> MNNSGTIETSQSVDRVTHKILIDGSEIPGTYQVKSIQVTKEVNRIPTARLVILDGDAAERDFKVSNSDHFVPGKEIEITVGYHSDDETIFKGVVIRQNLKIRNNQSILIVESRDMAVKMTLRRKSKYFYELSDSDILEELISNHGLEADVASTENQHTELVQYDVTDWDFMMLRLQANGLLCLVDDGKVSIQKPDLSSEALETVTFGATILEFDAEMDARNQLPKVVSQAWNMSDQELLEKEGVDPSLETNGNISSSDLASLFDQEEEVLRHGGSKKDGSLQEWANAK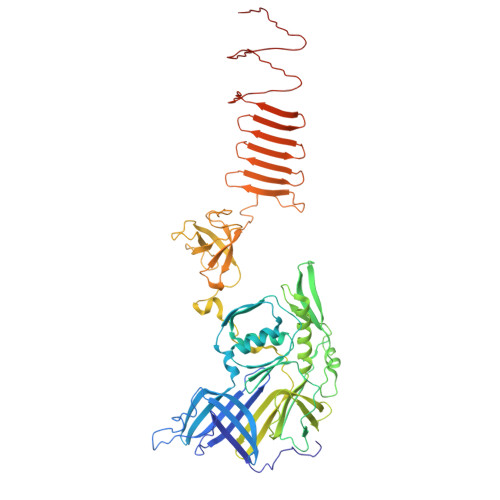WTFQQLAKTRGRIKFQGIPTVKPGVNLLLEGVGDRFNGKVFITGVNHQISEGNWTVDAQFGLNPEWFSESESNIHTPPAAGLTAAISGLHVGLVTDLEDPDGEDRIKVKIPIINNEEEGVWCRQAFPDAGNERGITFRPEIEDEVIVGFINEDPNDAVVLGMLHSSANPNPIEASNDNHEKGIQTRSGIKMIFNDEKSILQIETPTGNLVTLDDDAGSITIEDQNGNKTVMDSDGITMESAKDMNLKASGDINLEGTNVNIKANAEFKAEGSAGAEVSTSAVAVLKGSLVQIN> GSPEFEEQEAIMK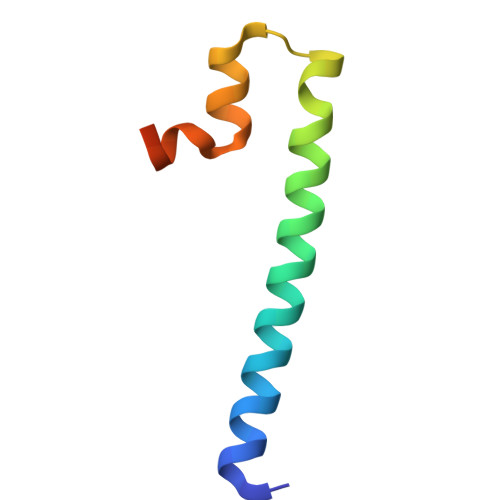VLQRDAALKRAEEERVRHLPEKIKDDQQLKNMSGQWFYEAKAKRHA>MTKPLIKPDVDLTDGNFYASRQAREAYRWMRANQPVFRDRNGLAAASTYQAVIDAERQPELFSNAGGIRPDQDALPMMIDMDDPAHLLRRKLVNAGFTRKRVKDKERSIAQLCDTLIDAVCERGECDFVRDLAAPLPMAVIGDMLGVLPEQREMFLRWSDDLVTFLSSHVSQEDFQVTIDAFAAYNDFTRATIAARRAEPTDDLVSVLVSSEVDGERLSDDELVMETLLILIGGDETTRHTLSGGSEQLLRNRDQWDLLQSDRELLPGAIEEMLRWTAPVKNM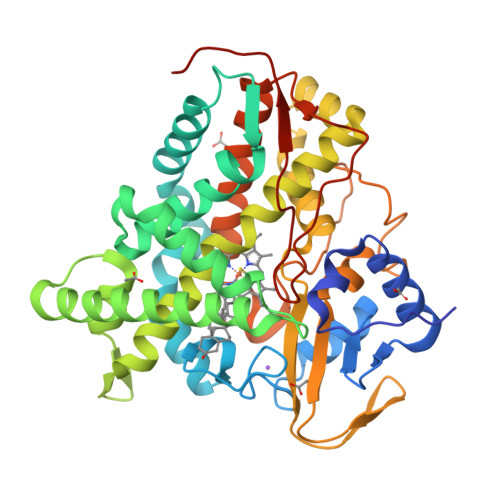CRMLTADTEFHGTALSEGEKIMLLFESANFDEAVFTDPEKFDIQRNPNSHLAFGFGTHFCMGNQLARLELSLMTARVVQRLPDLRLADQDSRLPLRPANFVSGLESMPVVFTPSRPLSGGSG[2x]>AECSVDIQGNDQMQFNTNAITVDKSCKQFTVNLSHPGNLPKNVMGHNWVLSTAADMQGVVTDGMASGLDKDYLKPDDSRVIAHTKL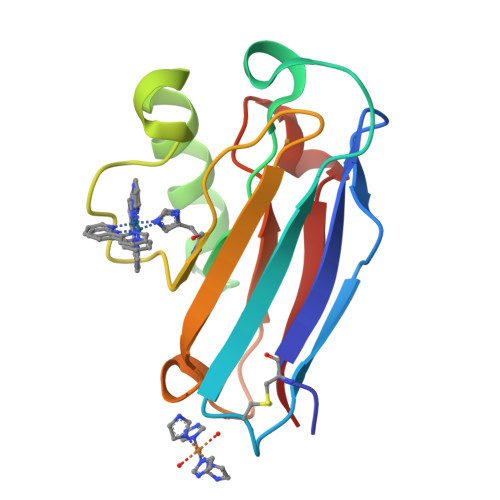IGSGEKDSVTFDVSKLKEGEQYMFFCTFPGHSALMKGTLTLK[2x]>DGVDIYFGMPGEISEHEGFLRAKMDLEERRMRQINEVMREWAMADNQSKNLPKADRQALNEHFQSILQTLEEQVSGERQRLVETHATRVIALINDQRRAALEGFLAALQADPPQAERVLLALRRYLRAEQKEQRHTLRHYQHVAAVDPEKAQQMRFQVHTHLQVIEERVNQSLGLLDQNPHLAQELRPQIQELLHSEHLGPSE[2x]

APP and its paralogues APP-like protein 1 (APLP1) and APP-like protein 2 (APLP2) contain the highly conserved heparan sulfate (HS) binding domain E2, which effects various (patho)physiological functions. The ectodomains of all APP-family proteins share the N-terminal E1 domain and the central E2 domain. Comparable to the E2 structures of other APP-family proteins, a coiled-coil-like fold is formed by helix αB (Gly302–Gln338) and the first half of helix αC (Lys344–Arg379). The C-terminal parts of helices αC (Val380–Leu399), αD (Ala406–Val437), αE (Pro439–Asp468) and αF (Pro471–Gly491) constitute a four-helix bundle.

We identified a new orthorhombic crystal form of the E2 domain of APLP1. The respective structure was built and refined to 2.6 Å resolution. Indeed, the N-terminal helix αA was not observed in the new crystal form (although it was present in the protein construct used), suggesting that it is rather flexible and becomes sufficiently stabilized only by certain intermolecular interactions. The apo structure of APLP1 E2 revealed an unfolded and hence flexible N-terminal helix αA. The folding of helix αA is shown to be independent of the other structural parts of APLP1 E2. A similar arrangement has been described for APLP1 E2 in previous studies and was functionally connected to heparin binding. Despite the similar overall topologies of these dimeric APLP1 E2 assemblies, the Cα r.m.s.d. value of approximately 1.5 Å (for helices αB7–αF) is rather large between the crystal structure described here and that solved previously. Beyond the differently structured N-terminal segments (N-terminal residues Asp292–Ile304), a high overall similarity of the heparin-bound and unbound APLP1 E2 structures was observed.Remarkably, the quality control system is equipped with an elaborate backup mechanism employing a molecular ‘gatekeeper’ that can specifically catalyse reglucosylation against incompletely folded glycoproteins as potential substrates, thereby regenerating monoglucosylated glycoforms for their return to the chaperone-assisted folding process. This gatekeeper function is executed by a unique enzyme, UDP-glucose:glycoprotein glucosyltransferase (UGGT). Our results reveal that UGGT has a modular structure in which the 35-kDa catalytic domain is tethered to the 125-kDa folding-sensor region. The N-terminal folding-sensor region is composed of the four Trx-like domains and the β-domain assembled into the C-shaped structure with structural plasticity harbouring the central cavity displaying hydrophobic patches, which putatively accommodates incompletely folded glycoproteins.

We determined the crystal structure at a 1.40-Å resolution of the C-terminal catalytic domain (CAT, residues 1190–1480) in complex with a UDP-glucose donor substrate and Ca2+, which are required for the enzymatic activity. In the CAZy classification, the CAT domain belongs to the GT24 family, which is supposed to share structural similarity with the GT8 family. This was confirmed by the present crystal structure showing a GT-A fold comprising nine β-strands and 12 α-helices. The UDP-glucose and Ca2+ ligands were accommodated in the active site containing a DXD motif (D1294-A1295-D1296), in which the ligand binding residues are essentially identical across species together with the retaining GT8 glycosyltransferases14, suggesting that the enzymatic mechanism of UGGT is evolutionarily conserved. In comparison with UDP-glucose-bound complex, 1379–1387 and 1427–1438 loops containing Asn1386 and Asn1430 located closer to the glucose- or Tris-binding site undergo significant structural changes upon UDP binding, suggesting its mechanism of release of the monoglucosylated product. In both crystal structures, a remarkable hydrophobic patch was found around the active site, implying its possible contribution to the folding-sensing mechanism of the catalytic domain.

> GSADINIFSVASGHLYERMLNIMMVSVMKHTKHSVKFWFIEQFLSPSFKKFLPHLAKEYGFSYEMVTYKWPHWLRGQREKQREIWGYKILFLDVLFPLSLDKVIFVDADQIVRTDMYDLVQLDLEGAPYGFTPMCDSRKEMEGFRFWKQGYWKSHLRGRPYHISALYVVDLNRFRALAAGDRLRGQYHTLSADPNSLANLDQDLPNNMQAMIPIKSLPQEWLWCETWCADEDLKTARTIDLCNNPLTKEPKLDRARRQVPEWTEYDNEIAELAVRVRAASKQSRREEDEKKDV> MNHKHHHHHHSSGLVPRGSAMGFDDKILLITGGTGSFGNAVMKRFLDSNIKEIRIFSRDEKKQDDIRKKYNNSKLKFYIGDVRDSQSVETAMRDVDYVFHAAALKQVPSCEFFPVEAVKTNIIGTENVLQSAIHQNVKKVICLSTDKAAYPINAMGISKAMMEKVFVAKSRNIRSEQTLICGTRYGNVMASRGSVIPLFIDKIKAGEPLTITDPDMTRFLMSLEDAVELVVHAFKHAETGDIMVQKAPSSTVGDLATALLELFEADNAIEIIGTRHGEKKAETLL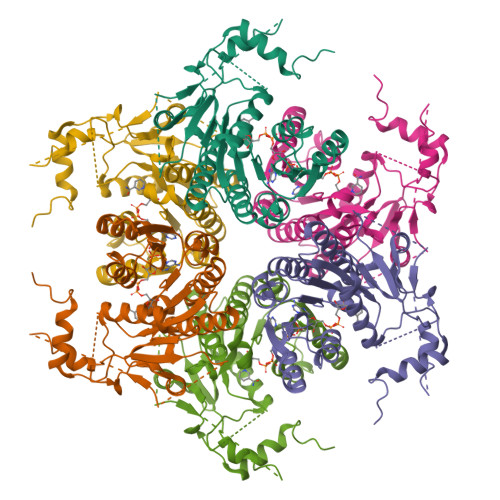TREEYAQCEDMGDYFRVPADSRDLNYSNYVETGNEKITQSYEYNSDNTHILTVEEIKEKLLTLEYVRNELNDYKASMR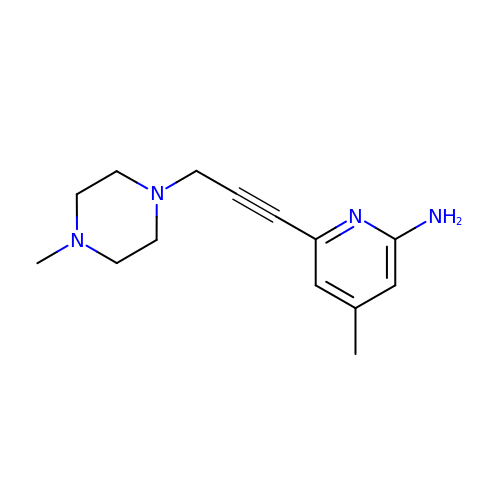4-methyl-6-[3-(4-methylpiperazin-1-yl)prop-1-yn-1-yl]pyridin-2-amine | C14 H20 N4 | VWGJRTCMKOXFHS-UHFFFAOYSA-N> GSGGGKPS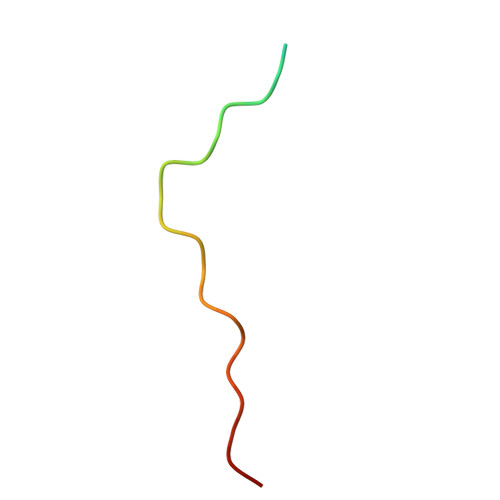RPPRPSRPPPPTPRRPASY>HMDDISQDNFLLSKEYENSLDVDTKKASGIYYTPKIIVDYIVKKTLKNHDIIKNPYPRILDISCGCGNFLLEVYDILYDLFEENIYELKKKYDENYWTVDNIHRHILNYCIYGADI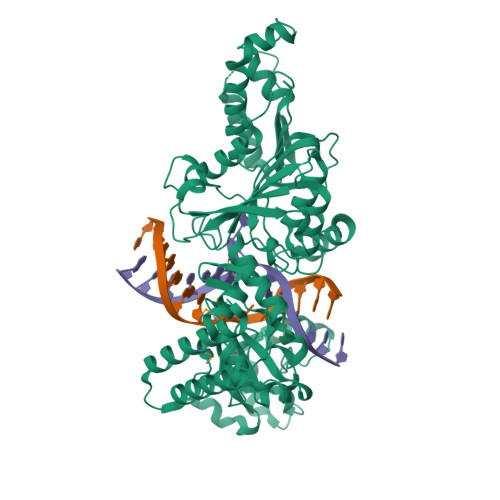DEKAISILKDSLTNKKVVNDLDESDIKINLFCCDSLKKKWRYKFDYIVGNPPYIGHKKLEKKYKKFLLEKYSEVYKDKADLYFCFYKKIIDILKQGGIGSVITPRYFLESLSGKDLREYIKSNVNVQEIVDFLGANIFKNIGVSSCILTFDKKKTKETYIDVFKIKNEDICINKFETLEELLKSSKFEHFNINQRLLSDEWILVNKDDETFYNKIQEKCKYSLEDIAISFQGIITGCDKAFILSKDDVKLNLVDDKFLKCWIKSKNINKYIVDKSEYRLIYSNDIDNENTNKRILDEIIGLYKTKLENRRECKSGIRKWYELQWGREKLFFERKKIMYPYKSNENRFAIDYDNNFSSADVYSFFIKEEYLDKFSYEYLVGILNSSVYDKYFKITAKKMSKNIYDYYPNKVMKIRIFRDNNYEEIENLSKQIISILLNKSIDKGKVEKLQIKMDNLIMDSLGI[3x]>MEFKDFPLKPEILEALHGRGLTTPTPIEAAALPLALEGKDLIGQARTGTGKTLAFALPIAERLAPSQERGRKPRALVLTPTRELALQVASELTAVAPHLKVVAVYGGTGYGKQKEALLRGADAV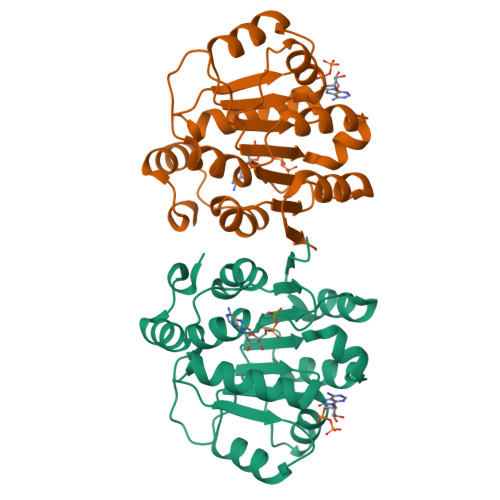VATPGRALDYLRQGVLDLSRVEVAVLDEADEMLSMGFEEEVEALLSATPPSRQTLLFSATLPSWAKRLAERYMKNPVLINVIK[4x]>[2x]MPSLTPRCIIVRHGQTEWSKS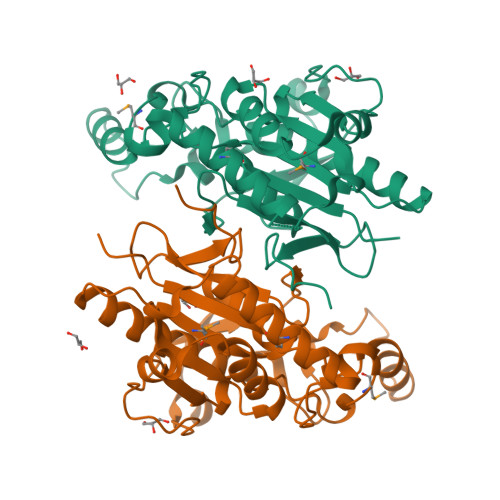GQYTGLTDLPLTPYGEGQMLRTGESVFRNNQFLNPDNITYIFTSPRLRARQTVDLVLKPLSDEQRAKIRVVVDDDLREWEYGDYEGMLTREIIELRKSRGLDKERPWNIWRDGCENGETTQQIGLRLSRAIARIQNLHRKHQSEGRASDIMVFAHGHALRYFAAIWFGLGVQKKCETIEEIQNVKSYDDDTVPYVKLESYRHLVDNPCFLLDAGGIGVLSYAHHNIDEPALELAGPFVSPPEGS>XGLLEEIAQLLEEIAKLLKKI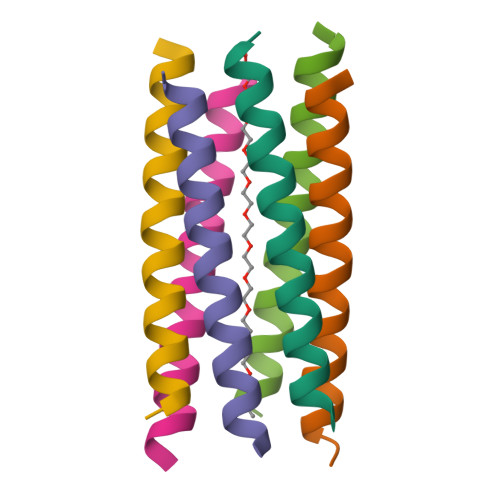AWLLKKIAQGX[6x]> SELIVNVINGPSLGRLGRREPAVYGGTTHDELVALIEREAAELGLKAVVRQSDSEAQL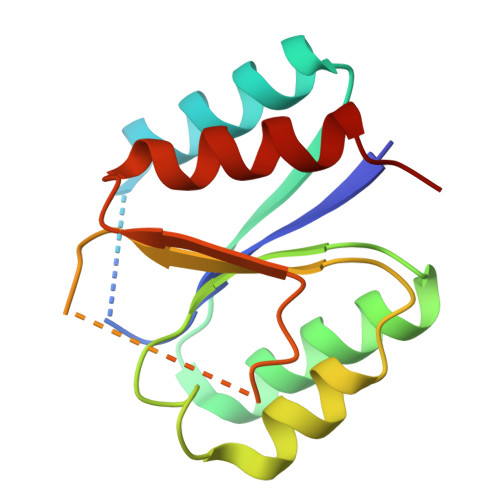LDWIHQAADAAEPVILNAGGLTHTSVALRDACAELSAPLIEVHISNVHAREEFRRHSYLSPIATGVIVGLGIQGYLLALRYLAEHLGT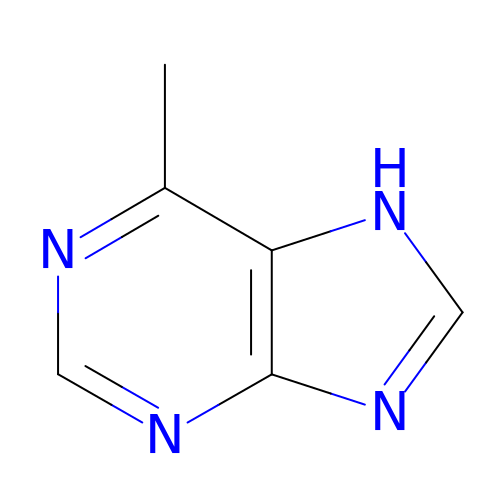6-METHYLPURINE | C6 H6 N4 | SYMHUEFSSMBHJA-UHFFFAOYSA-N>[2x]FSVEFKATENEIVSGKLDADTPAFHLVMSDSGEHKGWNVRPTGASEGGQMVSADGTRVDLHTNELSWDNDHWWI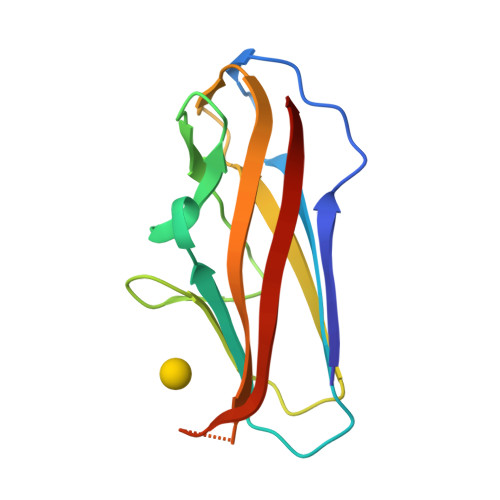DDGSERVEATFFLAAGDEVKAGEYQFTGRVEEYVEDNKQEPTVINSKDISATKTVKE>[4x]ADDPIRMYFEPGH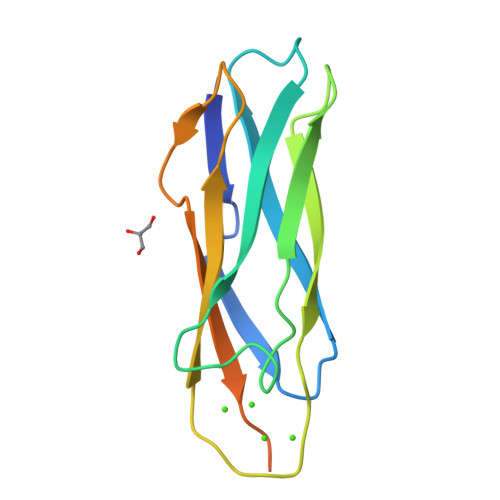YTVMENCGEFEVRVVRRGDISTYASVEYETQDGTASAGTDFVGRKGLLSFPPGVDEQRFRIEVIDDDVFEEDECFYIRLFNPSEGVKLAVPMIATVMILDDDHAGIFAFTDSVFEITESVGRFE> GAMDY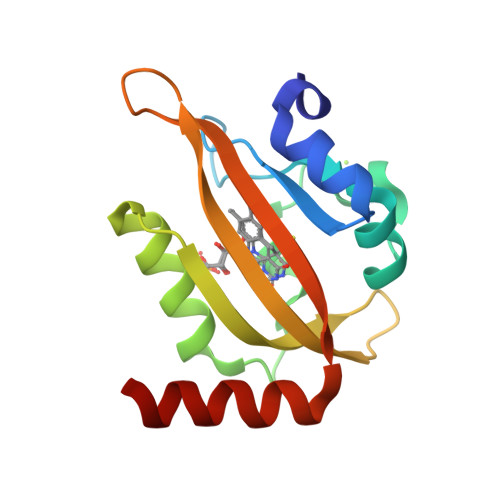SLVKALQTAQQNFVISDPSIPDNPIVYASQGFLTLTGYALSEVLGRNCRFLQGPETDPKAVEKVRKGLERGEDTTVVLLNYRKDGSTFWNQLFIAALRDGEGNVVNYLGVQCKVSEDYAKAFLKNEENEK>PGAIREDTPPGSVIQYSDYELDHSSPFAGGVAWIEGEFLPAEDAKISIFDTGFGHSDLTYTVAHVWHGNIFRLGDHLDRLLDGARKLRLDAGYTKDELADIT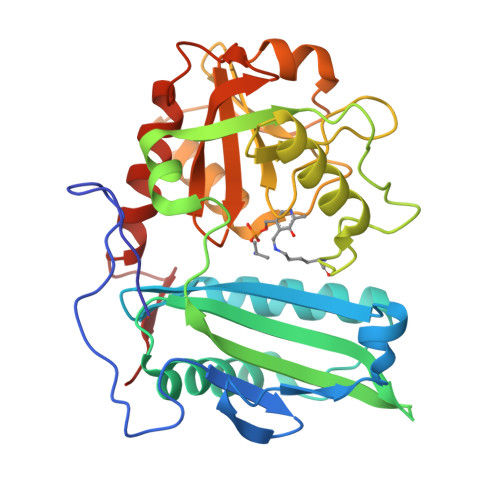KQCVSMSQLRESFVNLTVTRGYGKRRGEKDLSKLTHQVYIYAIPYLWAFPPAEQIFGTTAIVPRHVRRAGRNTVDPTIKNYQWGDLTAASFEAKDRGARTAILLDSDNCVAEGPGFNVCIVKDGKLASPSRNALPGITRKTVFEIADQMGIEATLRDVTSHELYDADELMAVTTAGGVTPINSLDGEAIGNGAPGPMTVAIRDRFWALMDEPGPLIEAIEY[4x]2-[2,5-bis(chloranyl)-1-benzothiophen-3-yl]ethanoic acid | C10 H6 Cl2 O2 S | 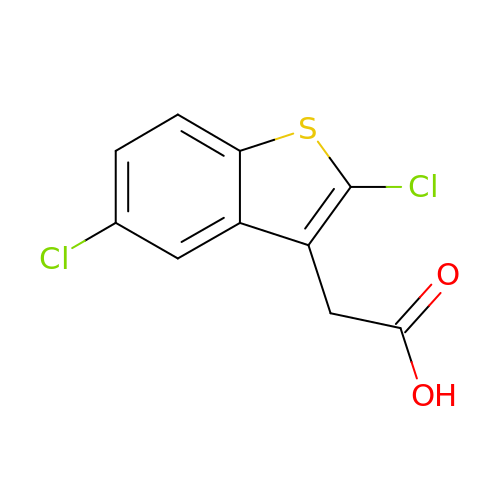BCQFHYKPVHGTMB-UHFFFAOYSA-N>[2x]SARSCTIHKEDLQDGLPVLIPKEDSLLYAGSVRTLQPPDIYSIVIEG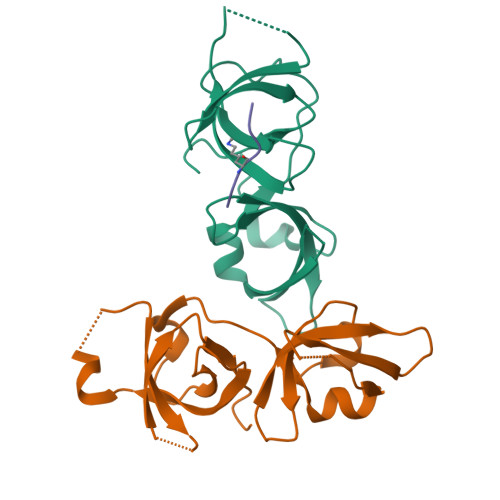ERGNRQRIYSLEQLLQEAVLDVQPQSSRYLPPGTRVCAYWSQKSRCLYPGNVVRGASSDEEDLDSVLVEFDDGDTGHIAVSNIRLLPPDFKIQC;> GAKRHRKVLRDN> SAKALIVYGSTTGNTEYTAETIARELADAGYEVDSRDAASVEAGGLFEGFDLVLLGCSTWGDDSIELQDDFIPLF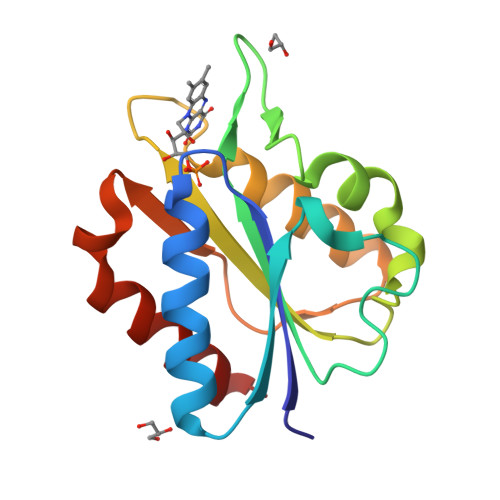DSLEETGAQGRKVACFGCGDSSWEYFCGAVDAIEEKLKNLGAEIVQDGLRIDGDPRAARDDIVGWAHDVRGAI> VVRPGS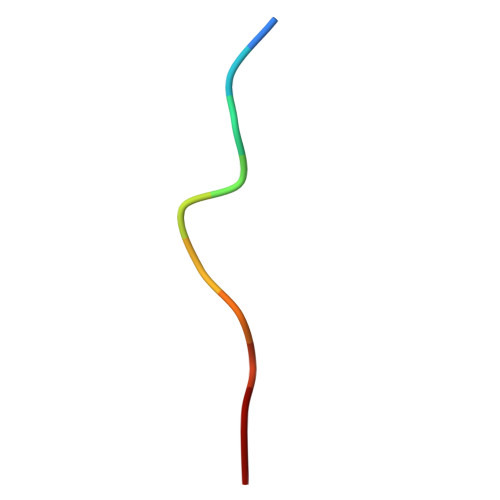LDLP> MSKVFAVYGASGCGRSLMPVANEQLRILEGDTDSQIVFIDDALDDNITVNGYTAMNYTKFKSIKNDDKFVLIAIANSSIRQKIADKLVKDGISLWTVQGMTTLIMDEVSIDAGAALSPFVTIAANVTIGKCFHANLYSYVEHDCIIGDYVTFAPRVSCNGNIHIHDHAYIGTGAVIKQGTPDKPLIIGKGAIVGMGAVV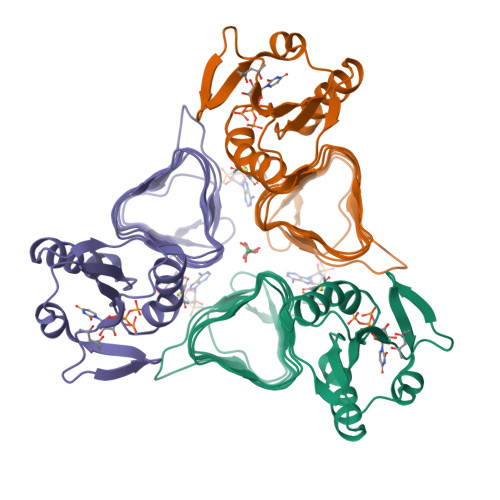TKEVPAGAVVIGNPARLLNKLEHHHHHH> GPHMTNIPQGMVTDQFGMIGLLTFIRAAET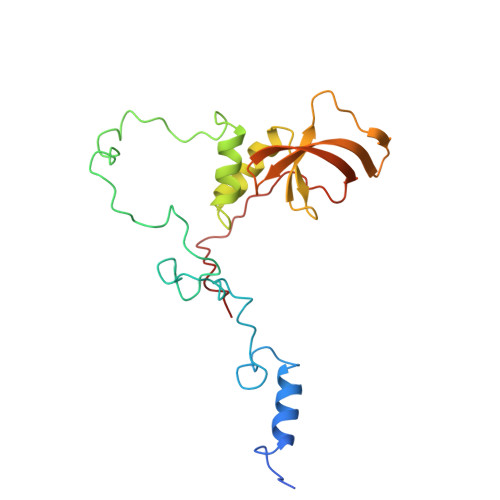DPGMVHLALGSDLTTLGLNLNSPENLYPKFASPWASSPCRPQDIDFHVPSEYLTNIHIRDKLAAIKLGRYGEDLLFYLYYMNGGDVLQLLAAVELFNRDWRYHKEERVWITRAPGMEPTMKTNTYERGTYYFFDCLNWRKVAKEFHLEYDKLEERPHLPSTFNYNPAQQAF> MVNKVLVANRGEIAVRIIRACKELGIPTVAIYNEVESTARHVKLADEAYMIGTDPLDTYLNKQRIINLALEVGADAIHPGYGFLAENAEFAKMCEEAGITFIGPHWKVIELMGDKARSKEVMKKAGVPVVPGSDGVLKSLEEAKALAREIGYPVLLKATAGGGGRGIRICRNEEELVKNYEQASREAEKAFGRGDLLLEKFIENPKHIEYQVLGDKHGNVIHLGERDCSIQRRNQKLVEIAPSLILTPEKREYYGNIVTKAAKEIGYYNAGTMEFIADQEGNLYFIEMNTRIQVEHPVSEMVTGIDIVKWQIKIAAGEPLTIKQEDVKFNGYAIECRINA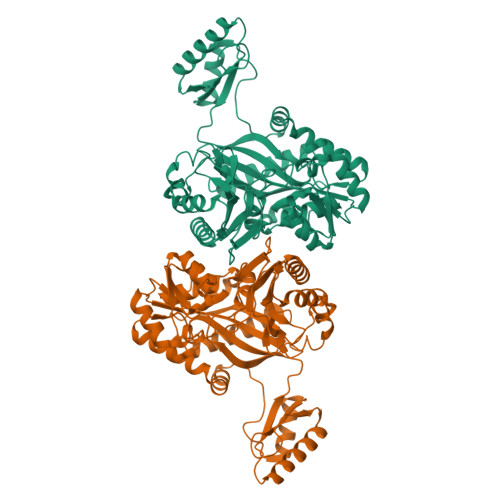EDPKKNFAPSTRVIERYYVPGGFGIRVEHAAARGFEVTPYYDSMIAKLITWAPTWDEAVERMRAALETYEITGVKTTIPLLINIMKEKDFKAGKFTTKYLEEHPEVFEYEE>HCDLPCGVYDPAQARIEAESVKAVQEKMAGNDDPHFQTRATVIKEQRAELAKHHVSVLWSDYFKPPHFEKYPELHQLVNDTLKAMSAAKGSKDPATGQKALDYIA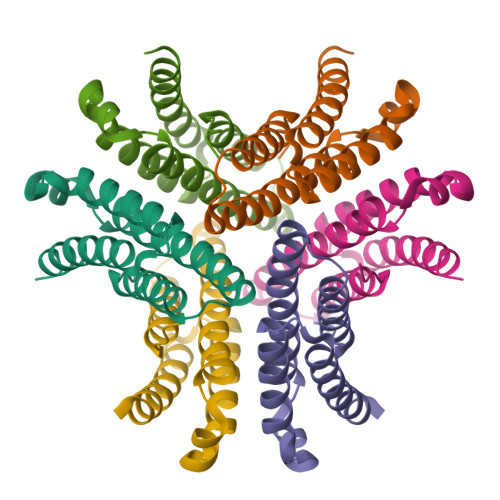QIDKIFWETKKA[3x]>APYINAAFRSSSEYEVYFFAKNKYVRLHYTPGASSDTILTNLRLISSGFPSLAGTPFAEPGIDCSFHTEASEAYVFSGNHSAYIDYAPGTTNDKILVGPTTIAEMFPVLNNTVFEDSIDSAFRSTKGKEVYLFK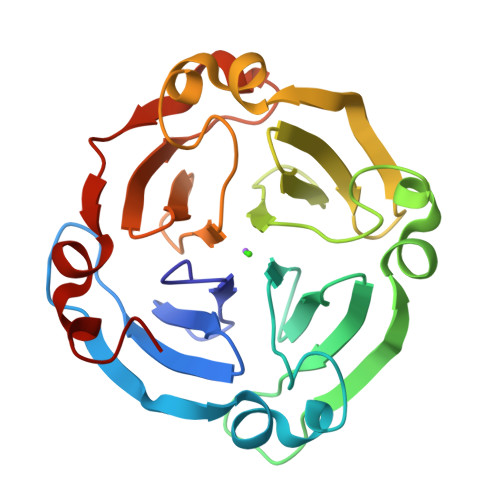GNKYVRIAYDSKQLVGNIRNIGDGFPVLNGTEFESGIDACFASHKEPEAYLFKGQNYVRIDFTPGGKADTLVGNIRPILDGWPVLKGIFPV[2x]> GCGGGCCCG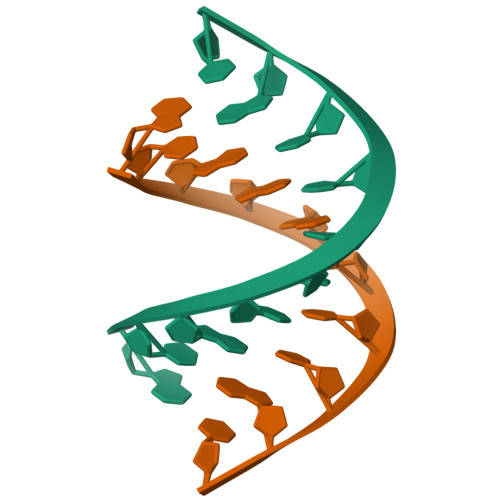C>MRVALLGGTGNLGKGLALRLATLGHEIVVGSRREEKAEAKAAEYRRIAGDASITGMKNEDAAEACDIAVLTIPWEHAIDTARDLKNILREKIVVSPLVPVSRGAKGFTYSSERSAAEIVAEVLESEKV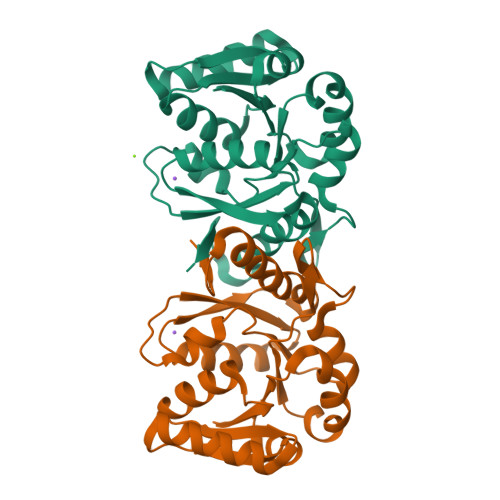VSALHTIPAARFANLDEKFDWDVPVCGDDDESKKVVMSLISEIDGLRPLDAGPLSNSRLVESLTPLILNIMRFNGMGELGIKFL[2x]>[2x]HGGEAHMVPMD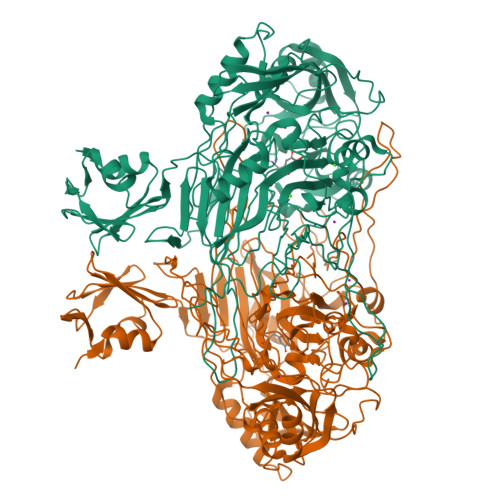KTLKEFGADVQWDDYAQLFTLIKDGAYVKVKPGAQTAIVNGQPLALQVPVVMKDNKAWVSDTFINDVFQSGLDQTFQVEKRPHPLNALTADEIKQAVEIVKASADFKPNTRFTEISLLPPDKEAVWAFALENKPVDQPRKADVIMLDGKHIIEAVVDLQNNKLLSWQPIKDAHGMVLLDDFASVQNIINNSEEFAAAVKKRGITDAKKVITTPLTVGYFDGKDGLKQDARLLKVISYLDVGDGNYWAHPIENLVAVVDLEQKKIVKIEEGPVVPVPMTARPFDGRDRVAPAVKPMQIIEPEGKNYTITGDMIHWRNWDFHLSMNSRVGPMISTVTYNDNGTKRKVMYEGSLGGMIVPYGDPDIGWYFKAYLDSGDYGMGTLTSPIARGKDAPSNAVLLNETIADYTGVPMEIPRAIAVFERYAGPEYKHQEMGQPNVSTERRELVVRWISTVGNYDYIFDWIFHENGTIGIDAGATGIEAVKGVKAKTMHDETAKDDTRYGTLIDHNIVGTTHQHIYNFRLDLDVDGENNSLVAMDPVVKPNTAGGPRTSTMQVNQYNIGNEQDAAQKFDPGTIRLLSNPNKENRMGNPVSYQIIPYAGGTHPVAKGAQFAPDEWIYHRLSFMDKQLWVTRYHPGERFPEGKYPNRSTHDTGLGQYSKDNESLDNTDAVVWMTTGTTHVARAEEWPIMPTEWVHTLLKPWNFFDETPTLGALKKDK>[2x]GNVDLVFLFDGSMSLQPDEFQKILDFMKDVMKKLSNTSYQFAAVQFSTSYKTEFDFSDYVKWKDPDALLKHVKHMLLLTNTFGAINYVATEVFREELGARPDATKVLIIITDGEATDS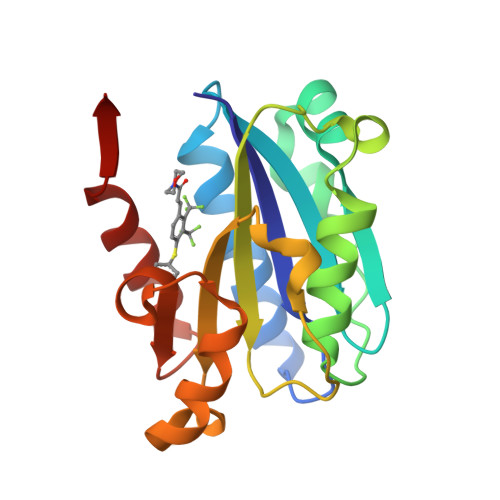GNIDAAKDIIRYIIGIGKHFQTKESQETLHKFASKPASEFVKILDTFEKLKDLFTELQKKIYVI> GCGTNGCGG;> 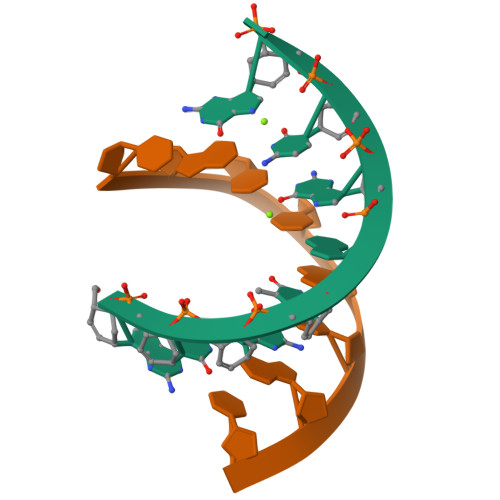CGCUACGC N'-[(E)-(2,4-dichlorophenyl)methylidene]-3,4-dihydroxybenzohydrazide | C14 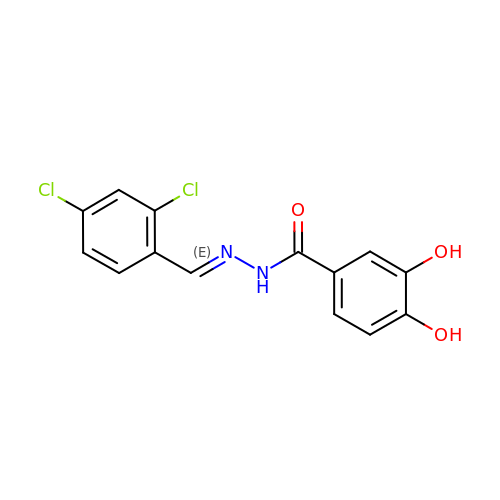H10 Cl2 N2 O3 | ISRFJSGSMHRMSJ-REZTVBANSA-N>DPLLPGYSFNAHLVAGLTPIEANGYLDFFIDRPLGMKGYILNLTIRGQGVVKNQGREFVCRPGDILLFPPGEIHHYGRHPEAREWYHQWVYFRPRAYWHEWLNWPSIFANTGFFRPDEAHQPHFSDLFGQIINAGQGE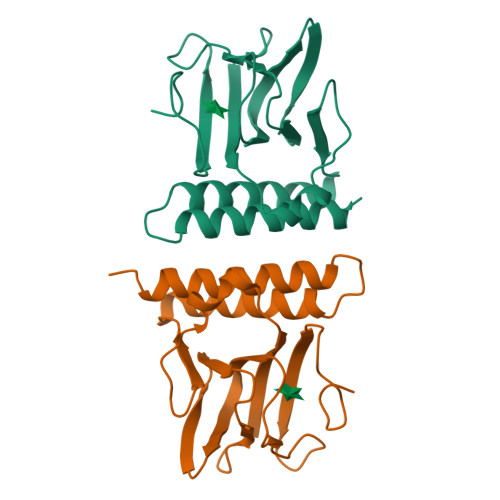GRYSELLAINLLEQLLLRRMEAINES[2x]> PEAPQPPAGLHWSWWELYVKGVNPEYPPRQRMFAFL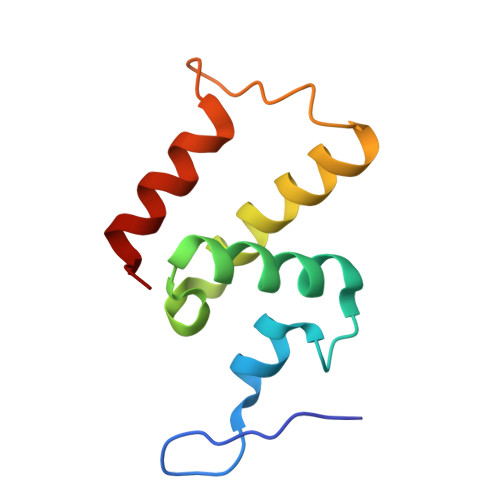TAQGVDVLEMEIREIEDVTRWLEMSNVYGEKFPRFPYDVTFQDKIEALKEKYPL>PHMKYYGNGVTCGKHSCSVDWGKATTCIINNGAMAW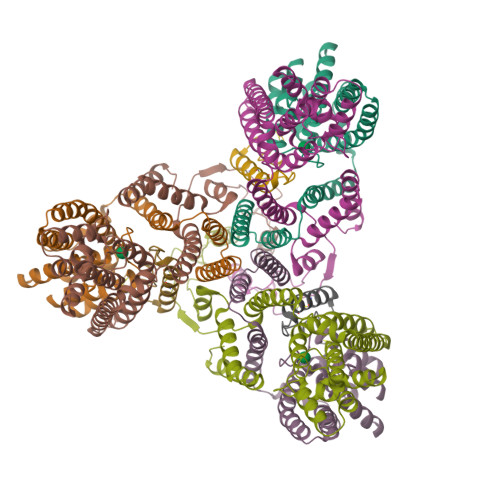ATGGHQGNHKC[3x];>[3x]MSVISIILVVLIAFLAGIEGILDEFQFHQPLIACTLIGLVTGNLTACIILGGTLQMIALGWANIGAAVAPDAALASVASAIILVLGGQGVAGIPSAIAIAIPLAVAGLFLTMIVRTLAVPIVHLMDRAAEKGNIRSVEWLHISAICMQGIRIAIPAAALLFIPADSVQSFLEAMPAWLTDGMAIGGGMVVAVGYALVINMMATKEVWPFFVIGFVVAAISQLTLIAIGALGVALALIYLNLSKMGGGNSNGGGGGNSRDPLGDILNDY;>[3x]MAEKIELSKRDRLRVAWRSTFIQGSWNYERMQNGGWAFSMIPAIKKLYKTKEDRSSALKRHLEFFNTHPYIASPILGVTLALEEERANGAEVDDVAIQGVKVGMMGPLAGVGDPVFWFTIRPMLGALGASLALSGNILGPILFFVAWNVIRWGFMWYTQEFGYKAGSKITDDLSGGLLQDITKGASILGMFVLAALVQRWVNIQFAPIISKVKLDEGAYIDWSHLPQGAQGIKTALQQQQAGLALSEIKVTTLQNNLDNLIPGLAAVALTFLCMWLLKKKISPIIIILGLFVVGIVGHLIGLL> MKHHHHHHSAGLEVLFQGPDSMQNQGSVSQGALNMRDQQAAAAENVTPERVWALWNEGNLFSLSLAQLQGFLSRCGVRTDPAAKKAAVVRQVEEYLHSKDTTVKGGGQGAASPQQHQQHGQQGGYGRWNQASVMQPETLLDLSQAGFYEGAANMVPKAFQLLVSDTAPDVVVSRVNTTAFPGFPSNTECYTLGASEKDVAIRSRYSKVLQWCCLNMSNLQMDGELYVDFGKLLLKPSVMRKNRRIVSSYTLQQRLQVNHPYTWVPTLPESCLSKIQEQFLQPEGFAPIGKGVQLTYSGTIKRSKDQLHVDLDNKGKVLAVNSAWVNLQTAWCTHAKGPDVRLLLRSRPPIRRQDVELFASTPIIKLADDDVADVLPPEHGQLVYLSEDETRLFERVSDRGVTITVREVKRQPLIILRDEEEDPRVEYSLSAHIPANAAKATDVRAVGLTAFELAGRLAGLVAEDFVREYGCEAKL;> MQSFSAAAPAASGDFSHITRNTVWGLWNEGNLFSLSVPELAFFLQEHCRVANVDPRAKKSALVRQVEEILSAEQQASATVPQEDNPHAIVVTDYDRAEDALEEADEYGDWGAEPGFEDRRELDFMELSPGRMGERYDPLSPRAFQLLHSETATDVGIASIDPSKLPGQSKVKNALAAIHVAPNDANKMRFRMAFEWCLMNIWNMNMPGELNIGAGKALYYRSVAKQNRNVMPLWTVQKHLYAQHPYAWFAIASESNVAAMESLAAALNMSIQQERTTSYKVTIRRMAEFFDCELNGQLKCTMMNKPWDRFFVS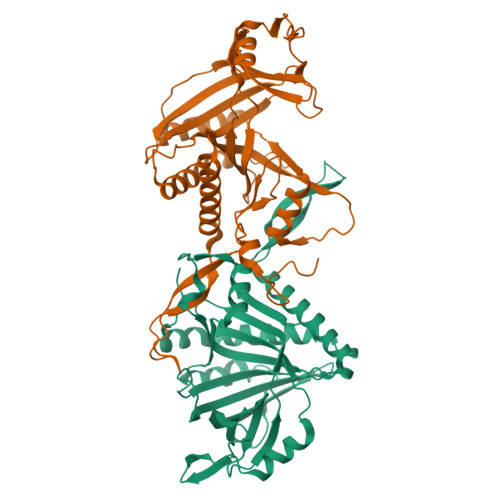HYIRSKMPDLRYVVRARHPIKKRIADAYLEADILRSTRDSVQSVLSPELGDVVYCCERVVRKWAKKTATGVTLQLVETKRTPLIITKAGDEGERLEYEWIVPLPQQAERIDIAALTDELWEYGNKLAAALEEGMEELMVHTMTAVSAY> HLSDMLQQLHSVNASKPSERGLVRQEEAEDPACIPIFWVSKWVDYSDKYGLGY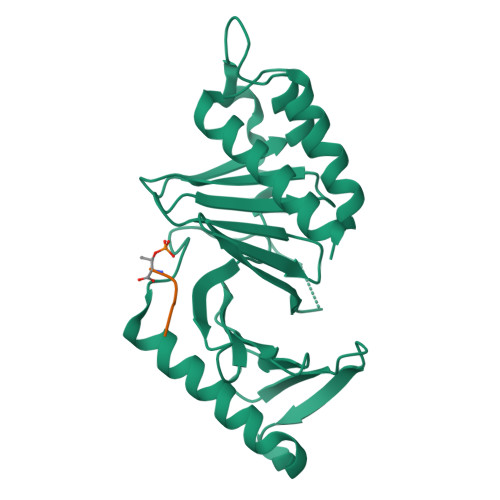QLCDNSVGVLFNDSTRLILYNDGDSLQYIERDGTESYLTVSSHPNSLMKKITLLKYFRNYMSEHLLKAGANITPREGDELARLPYLRTWFRTRSAIILHLSNGSVQINFFQDHTKLILCPLMAAVTYIDEKRDFRTYRLSLLEEYGCCKELASRLRYARTMVDKLLSS;> PPHST> GQRGWFCGSVSQDLRQFWVAEGGTISDPRAADFLFSCDASHPDTLRIYQSLDYIEDNATVFHAYYLSAVANAKIKNSVALGHFILPPACLQKEIRRKIGSFIWEQD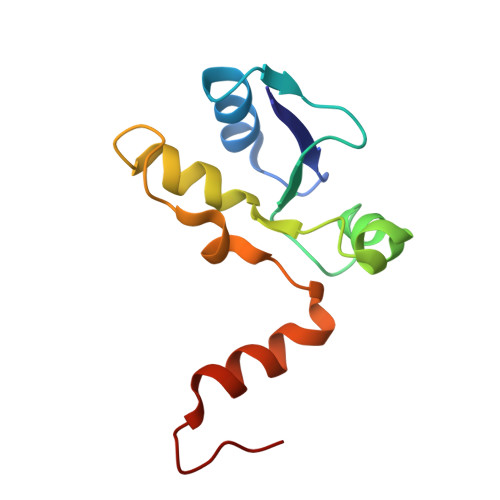Q>[6x]GPGSMSKRLRSSDVCADCNGPDPSWASVNRGTFI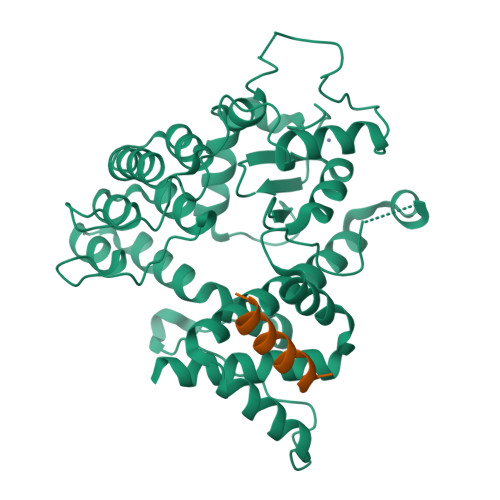CDECCSVHRSLGRHISQVRHLKHTAWPPTLLQMVETLYNNGANSIWEHSLLDPASIMSGRRKANPQDKVHPNKAEFIRAKYQMLAFVHRLPCREDDSVTAKDLSKQLHSSVRTGNLETCLRLLSLGAQANFFHPEKGSTPLHVASKAGQILQAELLAVYGADPGTQDSSGKTPVDYARQGGHHELAERLIEIQYELTDRLAFYLCGRKPDHKSGQHFLIPQRADAALDLSELAKAAKKKLQSLSNHLFEELAMDVYDEVDRRETDAVWLATQNHSTLVTETTVVPFLPVNPEYSSTRNQGRQKLARFNAHEFATLVIDILSDAKRRQQGS;>[6x]ALEEDAQILKVIEAYCTSAKT N-{4-[(2-benzyl-7-hydroxy-6-methoxyquinazolin-4-yl)amino]phenyl}benzamide | C29 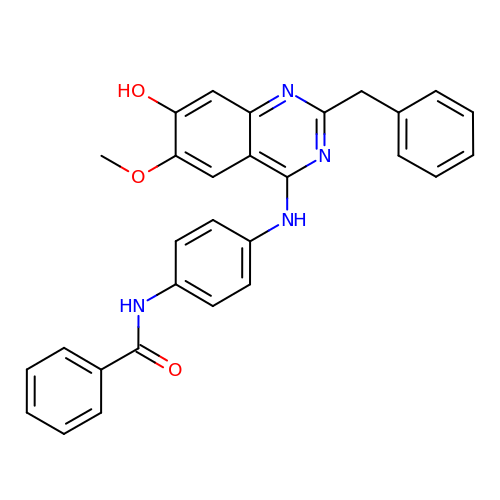H24 N4 O3 | MWYUDSZCUZWZIP-UHFFFAOYSA-N>[2x]GSHMLGLIKKKANTLLGIDISSTSVKLLELSRSGGRYKVEAYAVEPLPPN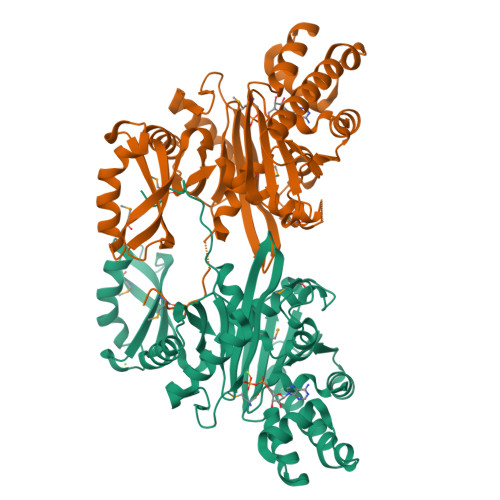AVVEKNIVELEGVGQALSRVLVKAKTNLKSAVVAVAGSAVITKTIEMEAGLSEDELENQLKIEADQYIPYPLEEVAIDFEVQGLSARNPERVDVLLAACRKENVEVREAALALAGLTAKVVDVEAYALERSYALLSSQLGADTDQLTVAVVDIGATMTTLSVLHNGRTIYTREQLFGGRQLTEEIQRRYGLSVEEAGLAKKQGGLPDDYDSEVLRPFKDAVVQQVSRSLQFFFAAGQFNDVDYIVLAGGTASIQDLDRLIQQKIGTPTLVANPFADMALNGKVNAGALASDAPALMIACGLALRSFD> GSARGPVGKRLQQELMTLMMSGDKGISAFPESDNLFKWVGTIHGAAGTVYEDLRYKLSLEFPSGYPYNAPTVKFLTPCYHPNVDTQGNICLDILKEKWSALYDVRTILLSIQSLLGEPNIDSPLNTHAAELWKNPTAFKKYLQETYSKQV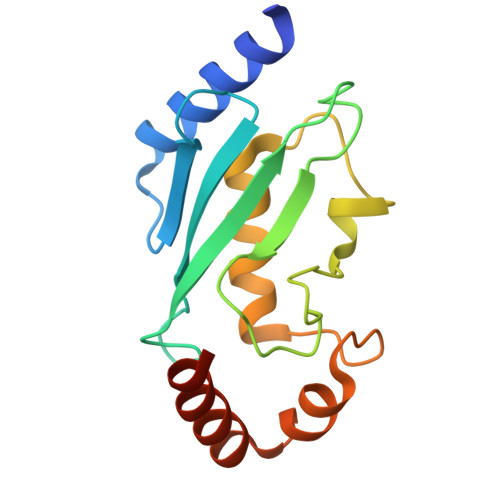TSQEP> MSSGKKPVKVKTPAGK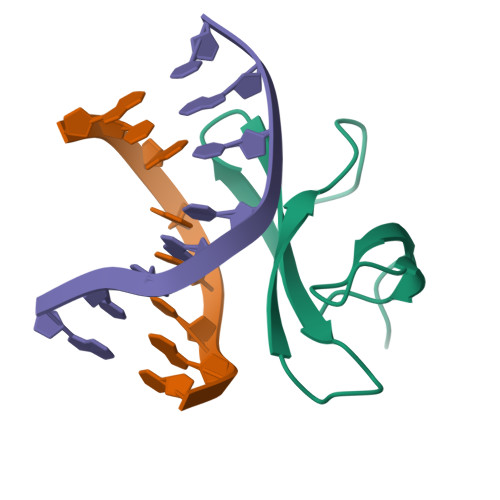EAELVPEKVWALGRVKIGLFKDPETGKYFRHKLPDDYPI> MQQGQMAYDRAITVFSPDGRLFQVEYAREAVKKGSTALGMKFANGVLLISDKKVRSRLIEQNSIEKIQLIDDYVAAVTSGLVADARVLVDFARISAQQEKVT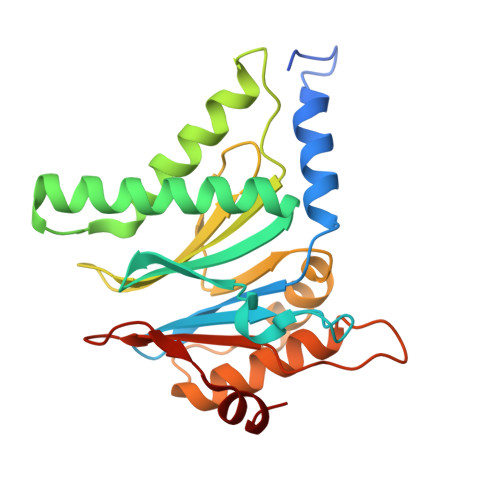YGSLVNIENLVKRVADQMQQYTQYGGVRPYGVSLIFAGIDQIGPRLFDCDPAGTINEYKATAIGSGKDAVVSFLEREYKENLPEKEAVTLGIKALKSSLEEGEELKAPEIASITVGNKYRIYDQEEVKKFL>[2x]YKWHYSGLNRWHGAGSTADFQKIIQERCDTYTQTIRPGSRSRNCQAIRQAFMSAFISKDPCKATKEDYNSLINLAPPTVPCGQQVFWSKTKELAHEYAKRRRLMTLEDTLLGYLAD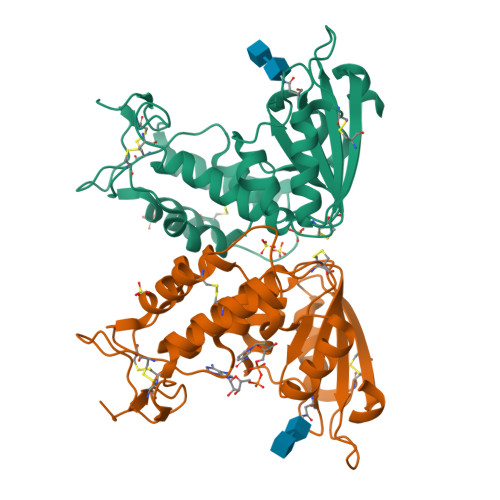GLRWCGEPGSSDLNIWSCPDWRKDCRTNYLSVFWEVLSERFAESACNTVRVVLNGSLENAFDSMSIFGRVQAPNLRPQVELEAWLVHDTGKPPSDSCSGSSIRKLKSILDGRNVKFRCMDNLSRDQFLQRS> KNDAEPVIDTDGNPLLHRGKYYIMPSNWGPPGGGLRLGKTRNLNCPVTVLQDYNEAINGLPVKFNIREILPRTIFTDTELN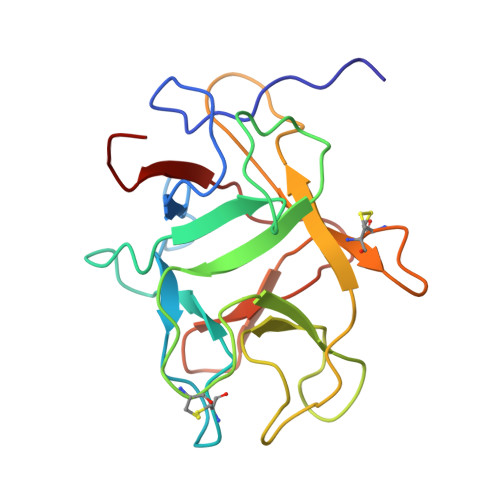IEFTEKPNCAENRAWSLFKGDDRGHKARVGIGGSNGHPGGEMLRGGFYGEQHGLRNGTYKLVFCRDGSSTCLDVGRYGNREGRRLGLSEAGELGVGFEKAGGGN>[2x]SNAMKKQEKLALVESALEDFYGDQQFASSLRESVLYSIHAGGKRIRPFLLLEVLEALQVTIKPAHAQVATALEMIHTGSLIHDDLPAMDDDDYRRGRLTNHKKFGEAMAILAGDALFLDSYALIAQADLPSQIKVDLIANLSLASGSLGMVAGQVLDMEGEHQHLSLEEL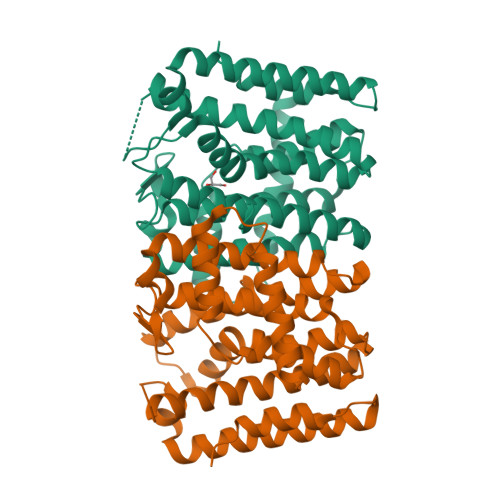QTIHANKTGKLLAYPFQAAAIIAELSPEMQVKLKTVGELIGLAFQVRDDVLDVTASFEEIGKTPQKDLQAEKSTYPALLGLEESIAFCNQTLDQANEKLEEIAQQLPFETESIVSVVESLRING Retention of α-Tol in animals requires α-tocopherol transfer protein (α-TTP) in the liver, a cytosolic transporter of 32 kDa weight. α-TTP belongs to the Sec-14 like family, a protein group involved in secretion and lipid transfer. α-TTP recognises and selectively extracts α-Tol from the endosomal fraction of the hepatocytes allowing for its transfer into the inner leaflet of the plasma membrane and eventually across the plasma membrane into the blood-stream. Here we show that, upon binding to α-Tol, α-TTP is formed acquiring tendency to aggregation into high molecular weight oligomers. X-ray diffraction reveals a spheroidal nanoparticle formed by 24 α-TTP protomers of ≈17 nm diameter. We verify that such particles are efficiently and selectively transported through a model endothelium tissue from human umbilical vein, with a 28-fold increased flux with respect to paracellular flux.

α-TTPS crystallised exclusively when starting from monodisperse solutions of monomeric α-TTP. α-TTPS can exist in different oxidation states; we obtained crystals in both the fully reduced and the fully oxidised states. X-ray diffraction patterns indicated that both crystals belong to the space group I432, with essentially identical unit-cell parameters a = 168.18 Å (reduced) and a = 168.26 Å (oxidised). The crystal structures were solved by molecular replacement method using the atomic model of monomeric α-TTP (PDB code 1OIP39) and refined at 2.40 Å resolution (reduced form; Rwork:Rfree 18.2%:21.5%) and at 2.42 Å resolution (oxidized form; Rwork:Rfree 19.1%:21.2%) respectively. In both cases, the asymmetric unit consists of a single α-TTP molecule (residues 48–278) with one α-Tol ligand bound to it. α-TTPS is formed by 24 protomers, for a molecular mass of 0.76 MDa, assembled into a spheroidal shell reminiscent of a viral capsid. The oxidised form of α-TTPS presents here one disulphide bridge crosslinking C80 of two α-TTP units through the rhombohedral channel. The oxidised α-TTPS particle thus contains a total of 12 S-S bridges covalently binding all trimeric subunits. Oxidation is accompanied by local unwinding of the helical segment (aa’s 65–79). It also induces structuring of the neighbouring C-terminus (aa’s 275–278) into a regular α-helical motif. We notice that folding stabilisation of the C-terminal amino acid residues accompanies the maturation of α-TTPS. In the oxidised α-TTPS, it is involved in a strong H-bond and salt-bridge network of interactions with the partner protein.

> TDSFLLRFLRARDFDLDLAWRLLKNYYKWRAECPEISADLHPRSIIGLLKAGYHGVLRSRDPTGSKVLIYRIAHWDPKVFTAYDVFRVSLITSELIVQEVETQRNGIKAIFDLEGWQFSHAFQITPSVAKKIAAVLTDSFPLKVRGIHLINEPVIFHAVFSMIKPFLTEKIKERIHMHGNNYKQSLLQHFPDILPLEYGGEEFSMEDICQEWTNFIMKSEDYLSSISESIQ9-ETHYL-9H-PURIN-6-YLAMINE | C7 H9 N5 | 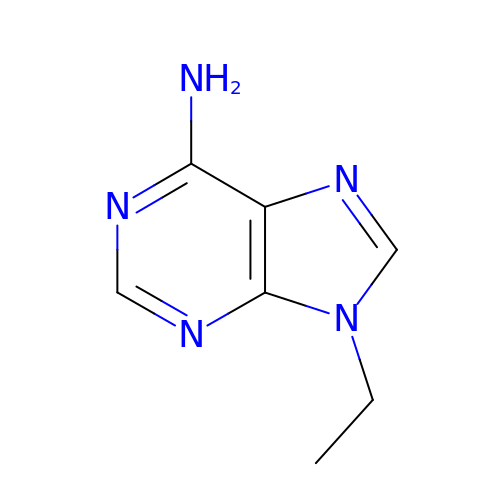MUIPLRMGAXZWSQ-UHFFFAOYSA-N> MKT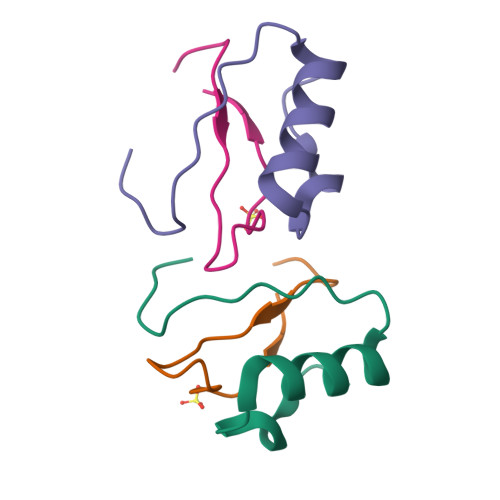EWPELVGKSVEEAKKVILQDKPEAQIIVLPVGTIVTMGQQQQGM;> EYRIDRVRLFVDKLDNIAQVPRVG>MKESLKDRIRLWKRLYVNAFENALNAIPNVKGVLLAYNTNIDAIKYLDADDLEKRVTEKGKEKVFEIIENPPEKISSIEELLGGILRSIKLGKAMEWFVESEEVRRYLREWGWDELRIGGQAGIMANLLGGVYRIPTIVHVPQNPKLQAELFVDGPIYVPVFEGNKLKLVHPKDAIAEEEELIHYIYEFPRGFQVFDVQAPRENRFIANADDYNARVYMRREFREGFEEITRNVELAIISGLQVLKEYYPDGTTYKDVLDRVESHLNILNRYNVKSHFEFAYTANRRV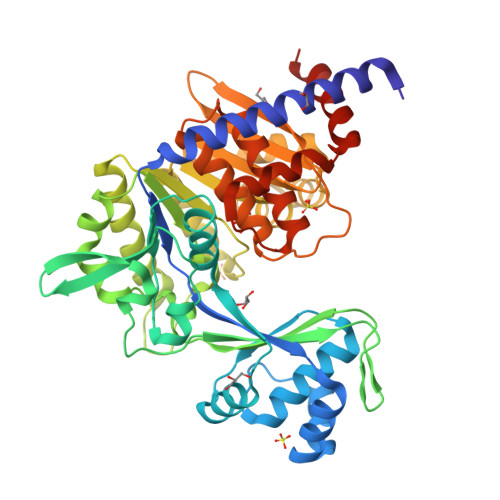REALVELLPKFTSVGLNEVELASIMEIIGDEELAKEVLEGHIFSVIDAMNVLMDETGIERIHFHTYGYYLALTQGGGRQLAFVPTKIVASPKSTVGIGDTISSSAFVSEFGGGGGVRDALLFASLAAAAKAMKGNLERIEQIRDALSVPTNERAIVLEEELEKEFTEFENGLIDMV[2x]>[8x]MALVVQKYGGSSLESAERIRNVAERIVATKKAGNDVVVVCSAMGDTTDELLELAAAVNPVPPAREMDMLLTAGERISNALVAMAIESLGAEAQSFTGSQAGVLTTERHGNARIVDVTPGRVREALDEGKICIVAGFQGVNKETRDVTTLGRGGSDTTAVALAAALNADVCEIYSDVDGVYTADPRIVPNAQKLEKLSFEEMLELAAVGSKILVLRSVEYARAFNVPLRVRSSYSNDPGTLIAGSMEDIPVEEAVLTGVATDKSEAKVTVLGISDKPGEAAKVFRALADAEINIDMVLQNVSSVEDGTTDITFTCPRSDGRRAMEILKKLQVQGNWTNVLYDDQVGKVSLVGAGMKSHPGVTAEFMEALRDVNVNIELISTSEIRISVLIREDDLDAAARALHEQFQLGGEDEAVVYAGTGR;>[8x]MEEAVLTGVATDKSEAKVTVLGISDKPGEAA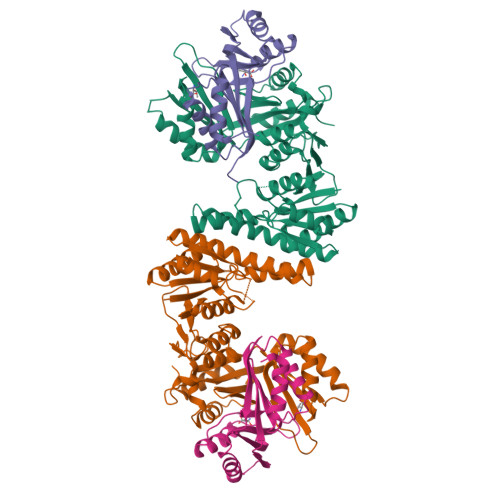KVFRALADAEINIDMVLQNVSSVEDGTTDITFTCPRSDGRRAMEILKKLQVQGNWTNVLYDDQVGKVSLVGAGMKSHPGVTAEFMEALRDVNVNIELISTSEIRISVLIREDDLDAAARALHEQFQLGGEDEAVVYAGTGRHHHHHH> GPHMASMLEAKFEEASLFKRIIDGFKKCVQLVNFQCKEDGIIAQAVDDSRVLLVSLEIGVEAFQEYRCDHPVTLGMDLTSLSKILRCGNNTDTLTLIADNTPDSIILLFEDTKKDRIAEYSLKLMDIDADFLKIEELQYDSTLSLPSSEFSKIVRDLSQLSDSINIMITKETIKFVADGDIGSGSVIIKPFVDMEHPETSIKLEMDQPVDLTFGAKYLLDIIKGSSLSDRVGIRLSSEAPALFQFDLKSGFLQFFLAPKFNDEE

PCNA is a ring-shaped homotrimeric complex that encircles DNA to act as a sliding clamp, ensuring processivity of DNA polymerases. It also operates as a platform for recruitment of numerous other proteins involved in DNA replication, DNA damage repair, mismatch repair, and chromatin structure and assembly. PCNA levels on DNA are regulated by loading and unloading. After completion of each Okazaki fragment, the Elg1 RFC-like complex (Elg1-RLC), which comprises the Elg1 subunit associated with the Rfc2–5 subunits, functions to unload PCNA from the lagging strand.

We then constructed strains expressing each PCNA mutant as the only copy of the POL30 gene, expressed from its endogenous locus, and found two PCNA mutants PCNA-D17K and PCNA-D21K that accumulate on DNA even with Elg1 present. Retention-prone mutants PCNA-D17K and PCNA-D21K have point mutations on the DNA-interacting region of inner ring. PCNA-D21K is unloaded from DNA slowly compared to WT PCNA, and is retained on DNA during S phase and even in G2/M phase. Elg1 can physically interact with PCNA-D17K and actually shows enhanced interaction with PCNA-D21K, suggesting that accumulation of those PCNA mutants on DNA is not due to a loss of interaction with the Elg1-RLC unloader. The structures (at 2.80- and 2.85-Å resolution for PCNA-D21K and PCNA-D17K, respectively) reveal that the mutations alter the inner pore of the PCNA ring. In both cases, the PCNA pore becomes more electropositive due to the swap of a negative charge to a positive charge. The D21K mutation positions lysine 21 to interact favorably in a bidentate manner with two backbone phosphates of DNA. For the D21K variant, we observed no significant conformational changes relative to wild-type PCNA (Cα RMSD ∼0.48 Å), indicating that the binding of PCNA partner proteins should not be perturbed. Our structural analysis and modeling indicates that the D21K variant strengthens direct interactions with the DNA backbone, without a substantial perturbation of the PCNA structure. The PCNA-D21K mutant provides an excellent tool for testing how PCNA retention on DNA affects cellular function.> MEGSNMETGQNLQNQPHTEVGTARPCRSCKWQTPDPTDPHRGQCTANRHAMGGVWKRWLRD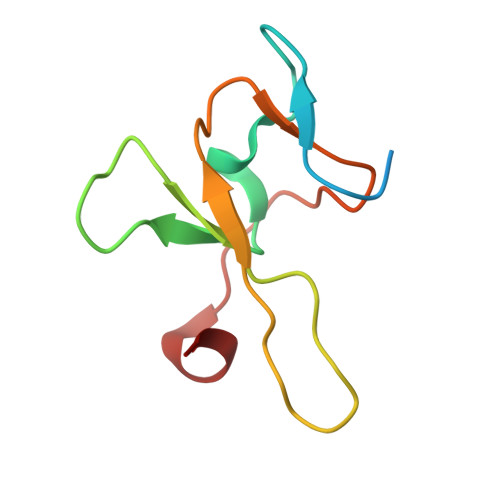VENTTCSRHEEGKLSFRDHV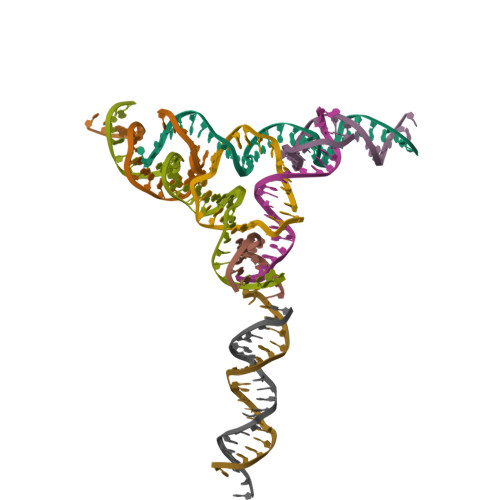> CAAGAGCCTGATCGGACAAGCGACGCAAGCA;> GAGCAGCCTGTACGGACATCA;> AACCTACCTGGCAGGACGACTCACTATGCTA;> TGTGCTTGCGTCGCTTGTGGCTGC;> TTTAGCATAGTGAGTCGTGGCTCT;> ACTGATGTGGTAGG;> TACACCGATCACCTGCCACCG;> GTCTCTGCTACTACGTCAGCA;> TCTGCTGACGTAGTAGCAGAG>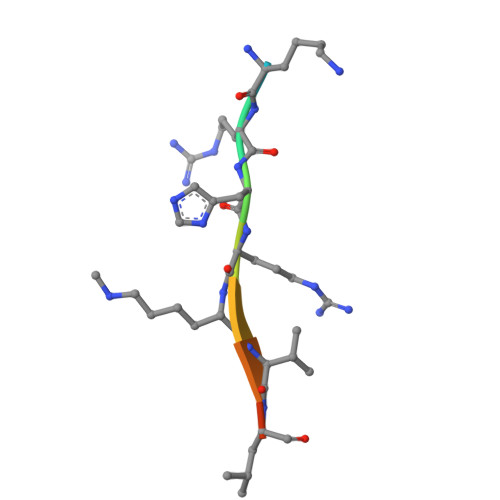 AKRHRKVLRD>[4x]MSLKDMIDSIEQFAQTQADFPVYDCL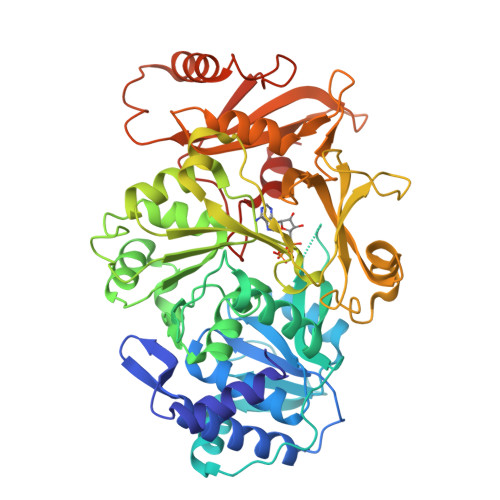GERRTYGQLKRDSDSIAAFIDSLALLAKSPVLVFGAQTYDMLATFVALTKSGHAYIPVDVHSAPERILAIIEIAKPSLIIAIEEFPLTIEGISLVSLSEIESAKLAEMPYERTHSVKGDDNYYIIFTSGTTGQPKGVQISHDNLLSFTNWMIEDAAFDVPKQPQMLAQPPYSFDLSVMYWAPTLALGGTLFALPKELVADFKQLFTTIAQLPVGIWTSTPSFADMAMLSDDFCQAKMPALTHFYFDGEELTVSTARKLFERFPSAKIINAYGPTEATVALSAIEITREMVDNYTRLPIGYPKPDSPTYIIDEDGKELSSGEQGEIIVTGPAVSKGYLNNPEKTAEAFFTFKGQPAYHTGDIGSLTEDNILLYGGRLDFQIKYAGYRIELEDVSQQLNQSPMVASAVAVPRYNKEHKVQNLLAYIVVKDGVKERFDRELELTKAIKASVKDHMMSYMMPSKFLYRDSLPLTPNGKIDIKTLINEVNNREGHHHHHH(2S)-2-[(N-acetyl-L-alpha-aspartyl)amino]nonanoic acid | 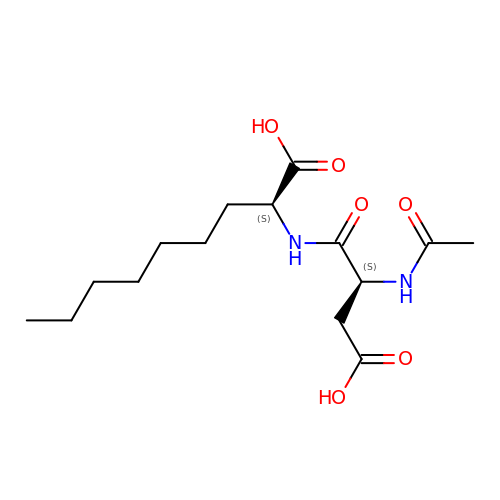C15 H26 N2 O6 | IRKQLRPKWIMPEM-RYUDHWBXSA-N>MKKEVCSVAFLKAVFAEFLATLIFVFFGLGSALKWPSALPTILQIALAFGLAIGTLAQALGPVSGGHINPAITLALLVGNQISLLRAFFYVAAQLVGAIAGAGILYGVAPLNARGNLAVNALNNNTTQGQAMVVELILTFQLALCIFASTDSRRTEPVGSPALSIGLSVTLGHLVGIYFTGCSMNPARSFGPAVVMNRFSPAHWVFWVGPIVGAVLAAI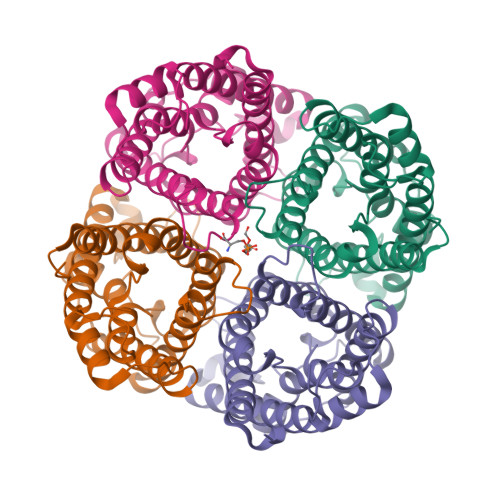LYFYLLFPNSLSLSERVAIIKGTYEP[8x]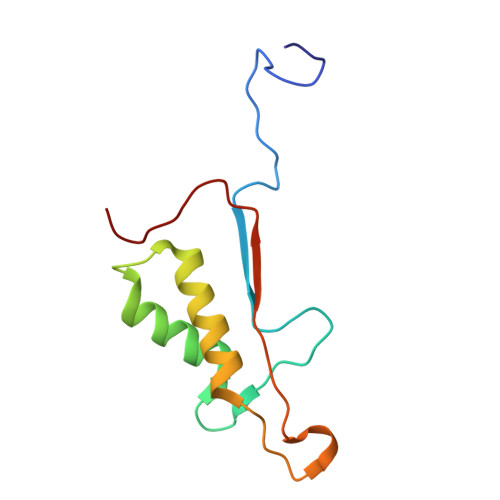> ASGVDDDMACHKIPVEADFLYAYSTAPGYYSWRNSKDGSWFIQSLCAMLKQYADKLEFMHILTRVNRKVATEFESFSFDATFHAKKQIPCIVSMLTKELYFYH1-[(benzyloxy)methyl]-6-(cyclohexylmethyl)-3-hydroxy-5-(propan-2-yl)pyrimidine-2,4(1H,3H)-dione | C22 H30 N2 O4 | 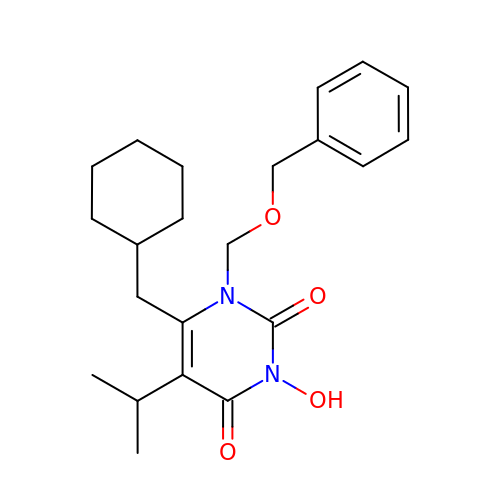ROZLWEMOPMWULZ-UHFFFAOYSA-N>NLYFQGHM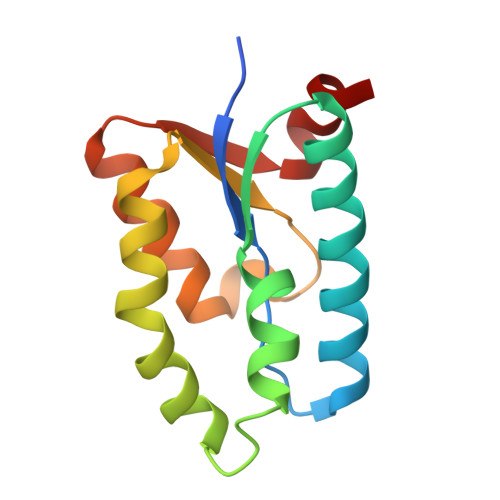RKIFLACPYSHADAEVVEQRFRACNEVAATIVRAGHVVFSQVSMSHPINLCLAELDRAAIGRLWAPVDAFYMDHLEELIVLDLPGWRDSAGIRREMEFFEAGGQRVSLWSEVEHEFR[2x]BAR protein endophilin B1 plays a key role in multiple cellular processes critical for oncogenesis, including autophagy and apoptosis. Endophilins are a highly conserved group of N-BAR proteins that contain an N-terminal amphipathic helix (H0) and a 20-residue amphipathic insert in helix 1 (H1i). These two motifs contribute to membrane association. BAR proteins are typically dimers in solution, where the dimer consists of three α-helices from each monomer that form a 6-helix bundle with a characteristic crescent shape.

Dimers bound to the surface of the bilayer and dimers that straddle the edges of the bicelle have distinct amphipathic helix conformations. These different classes of dimers will be referred to as “center” and “side” dimers, respectively. In center dimers, H1i is predominantly disordered. At lower contour levels the disordered region appears close to the BAR domain, brushing the membrane surface, but not inserted. H0s are oriented anti-parallel in relation to each other. As H1i is disordered in the center dimer class, residues Glu76-Ile96 were deleted from the model. Locally refining the classes individually resulted in reconstructions of 3.45 Å (center dimer) and 3.60 Å (side dimer), respectively. The atomic models consist of residues Leu11–Leu252. Residues Met1-Lys10 of H0 were omitted as weak density indicates that the N-terminus is flexible while inserted into the membrane. As the bicelle becomes more elliptical, the center dimers H0s move closer together, and the membrane density becomes more distinct.

>MNIMDFNVKKLAADAGTFLSRAVQFTEEKLGQAEKTELDAHLENLLSKAECTKIWTEKIMKQTEVLLQPNPNARIEEFVYEKLDRKAPSRINNPELLGQYMIDAGTEFGPGTAYGNALIKCGETQKRIGTADRELIQTSALNFLTPLRNFIEGDYKTIAKERKLLQNKRLDLDAAKTRLKKAKAAETRNSSEQELRITQSEFDRQAEITRLLLEGISSTHAHHLRCLNDFVEAQMTYYAQCYQYMLDLQKQLGSFPSNYLSNNNQTSVTPVPSVLPNAIGSSAMASTSGLVITSPSNLSDLKECSGSRKARVLYDYDAANSTELSLLADEVITVFSVVGMDSDWLMGERGNQKGKVPITYLELLN[2x]> SMASKNNIFNKYPTIIHGEARGENDEFVVHTRYPRFLARKSFDDNF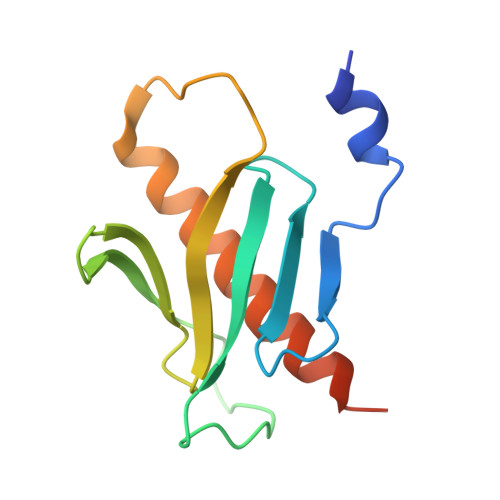TGEMPAKPVNGELGQIGEPRRLAYDSRLGLWLSDFIMLDNNKPKNMEDWLGQLKAACDRIAADDLMLNEDAADLEGWDD>AVDFSAHPWKAPGPNDSRGPCPGLNTLANHGFLPRNGRNISVPMIVKAGFEGYNVQSDILILAGKVGMLTSREADTISLEDLKLHGTIEHDASLSREDVAIGDNLHFNEAIFTTLANSNPGADVYNISSAAQVQHDRLADSVARNPNVTNTDLTATIRSSESAFYLTVMSAGDPLRGEAPKKFVNVFFQEERMPIKEGWKRSTTPINLPLLGPIIDRITELSDWKPTGDNCGAIVLGPGL[2x]

Here, we introduce a close ortholog of MroUPO, a UPO gene from Marasmius wettsteinii (MweUPO-1), that has a similar reaction profile to MroUPO and for which we have set up a directed evolution platform based on tandem-yeast expression. As a member of the heme-thiolate-containing peroxidase superfamily, UPO activity is fueled simply by H2O2, which plays a dual role of oxygen donor and final electron acceptor. In general terms, long UPOs are monomeric proteins with a molecular weight of ∼44 kDa and with a strong preference toward small aromatic compounds due to their narrower and “carafe-shaped” heme channel (e.g., AaeUPO vide infra). By contrast, short UPOs are either dimeric or monomeric proteins with a molecular size of ∼26 kDa per monomer, harboring a wide open and symmetric cone-shaped channel (frustum) that dictates their preference for bulky substrates like steroids and long aliphatic compounds (a preference attributed to MroUPO, see below). Here we present a new dimeric short UPO that can be heterologously expressed at high levels in both S. cerevisiae and P. pastoris, an enzyme that shares its substrate profile, selectivity, and biochemical and overall structural characteristics with MroUPO.

Long-chain substrates, alkanes (dodecane and tetradecane), and fatty acids (myristic acid and lauric acid) have a conserved “buried” mode of binding in close proximity to the heme. This type of binding maximizes the hydrophobic interactions between the main part of their corresponding chains to multiple residues establishing the contour of the heme channel (Ile55, Leu58, Val62, Thr152, Ile153). It seems apparent that these hydrophobic interactions govern the binding mode shared by all of these ligands, as the two alkanes fail to establish a polar link to MweUPO-1 residue Glu157 made by the carboxylate of the fatty acids. Indeed, while most UPOs can hydroxylate fatty acids, mainly at the ω1/ω2 positions, the progressive one-carbon shortening of mono- and dicarboxylic acids is a feature exclusively observed for MroUPO and MweUPO-1. Here, the captured lauric acid confirms this capacity, with its carboxylate coming into close contact with the heme and enabling shortening. As such, the results obtained by soaking MweUPO-1 crystals in lauric or myristic acid may be explained by the dependence on chain length described for monocarboxylic fatty acid shortening by MroUPO.>MSAKAISEQTGKELLYKFICTTSAIQNRFKYARVTPDTDWARLLQDHPWLLSQNLVVKPDQLIKRRGKLGLVGVNLTLDGVKSWLKPRLGQEATVGKATGFLKNFLIEPFVPHSQAEEFYVCIYATREGDYVLFHHEGGVDVGDVDAKAQKLLVGVDEKLNPEDIKKHLLVHAPEDKKEILASFISGLFNFYEDLYFTYLEINPLVVTKDGVYVLDLAAKVDATADYICKVKWGDIEFPPPFGREAYPEEAYIADLDAKSGASLKLTLLNPKGRIWTMVAGGGASVVYSDTICDLGGVNELANYGEYSGAPSEQQTYDYAKTILSLMTREKHPDGKILIIGGSIANFTNVAATFKGIVRAIRDYQGPLKEHEVTIFVRRGGPNYQEGLRVMGEVGKTTGIPIHVFGTETHMTAIVGMALGHRPIPNQPPTAAHTANFLLNASGSTSTPAPSRTASFSESRADEVAPAKKAKPAMPQDSVPSPRSLQGKSTTLFSRHTKAIVWGMQTRAVQGMLDFDYVCSRDEPSVAAMVYPFTGDHKQKFYWGHKEILIPVFKNMADAMRKHPEVDVLINFASLRSAYDSTMETMNYAQIRTIAIIAEGIPEALTRKLIKKADQKGVTIIGPATVGGIKPGCFKIGNTGGMLDNILASKLYRPGSVAYVSRSGGMSNELNNIISRTTDGVYEGVAIGGDRYPGSTFMDHVLRYQDTPGVKMIVVLGEIGGTEEYKICRGIKEGRLTKPIVCWCIGTCATMFSSEVQFGHAGACANQASETAVAKNQALKEAGVFVPRSFDELGEIIQSVYEDLVANGVIVPAQEVPPPTVPMDYSWARELGLIRKPASFMTSICDERGQELIYAGMPITEVFKEEMGIGGVLGLLWFQKRLPKYSCQFIEMCLMVTADHGPAVSGAHNTIICARAGKDLVSSLTSGLLTIGDRFGGALDAAAKMFSKAFDSGIIPMEFVNKMKKEGKLIMGIGHRVKSINNPDMRVQILKDYVRQHFPATPLLDYALEVEKITTSKKPNLILNVAGLIGVAFVDMLRNCGSFTREEADEYIDIGALNGIFVLGRSMGFIGHYLDQKRLKQGLYRHPWDDISYVLPEHMSM[4x]

ATP citrate lyase (ACLY) is the predominant nucleocytosolic source of acetyl-CoA and is aberrantly regulated in many diseases making it an attractive therapeutic target. Structural studies of ACLY reveal a central homotetrameric core citrate synthase homology (CSH) module flanked by acyl-CoA synthetase homology (ASH) domains, with ATP and citrate binding the ASH domain and CoA binding the ASH-CSH interface to produce acetyl-CoA and oxaloacetate products. The specific catalytic role of the CSH module and an essential D1026A residue contained within it has been a matter of debate. Here, we report biochemical and structural analysis of an ACLY-D1026A mutant demonstrating that this mutant traps a (3S)-citryl-CoA intermediate in the ASH domain in a configuration that is incompatible with the formation of acetyl-CoA, is able to convert acetyl-CoA and OAA to (3S)-citryl-CoA in the ASH domain, and can load CoA and unload acetyl-CoA in the CSH module.

To determine how the ACLY-D1026A mutant engages substrates, we preincubated ACLY-D1026A with substrates (citrate, CoA, and ATP) in an attempt to capture a reacted state of the mutant enzyme for cryo-EM structure determination. The cryo-EM structure (ACLY-D1026A—substrates) was determined at an overall resolution of 2.2 Å with imposing D2 symmetry. Unexpectedly, we observed unaccounted for cryo-EM density against the CSH domain that could be modeled as an additional CoA molecule bound in a previously unobserved “non-canonical” conformation, with the ADP group sitting near the center of the CSH module and the thioester of CoA pointing towards the end of the CSH module and bound in a ‘hole’ that is created by the removal of Asp1026. Notably, Arg 976, which plays an important role in binding non-productive, CoA changes position to avoid a steric clash with the binding of non-canonical CoA. The non-canonical CoA molecule bound to the CSH domain of the ACLY-D1026A—substrates structure sits across two subunits of the tetrameric CSH module (composed of four CSH domain subunits) such that it forms hydrophobic interactions with one CSH domain subunit and hydrogen bonds with the other CSH domain subunit, potentially locking the CSH module in a “closed” conformation that would not accommodate a translocated product from the ASH domain. In addition, a translocated product from the ASH domain would have to displace the non-canonical CoA molecule bound to the CSH domain. It therefore appears that the non-canonical CoA serves to trap (3 S)-citryl-CoA within the ASH domain. Interestingly, the loop containing His760 is disordered in the ACLY-D1026A—substrates structures, even though phosphate in the form of ATP was added in the ACLY-D1026A—substrates structure.> MLDRLDAALRFQQEALNLRAQRQEILAANIANADTPGYQARDIDFASELKKVMVRGREE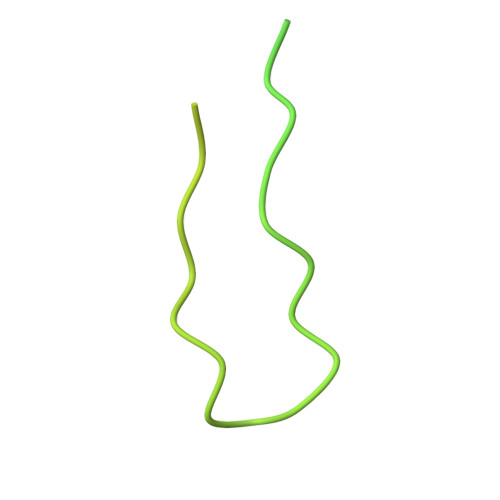TGGVALTLTSSHHIPAQAVSSPAVDLLYRVPDQPSLDGNTVDMDRERTQFADNSLKYQMGLTVLGSQLKGMMNVLQGGN> GMNLANIV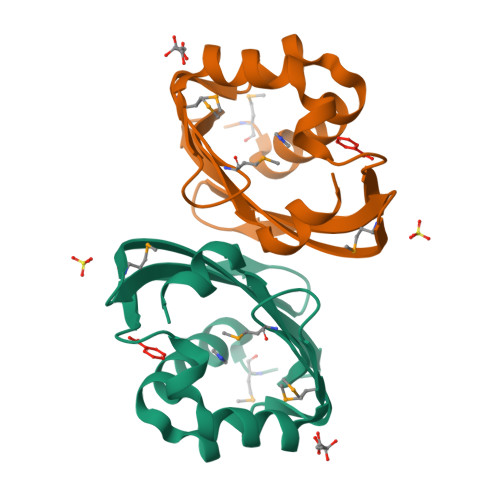QRGWEALGAGDFDTLVTDYVEKMIFIMPGQADVLKGRQAFRSALDNLGEILPPGFEITGLRQLEGENEIVSIVEWKSDKMIASQLSVLFKFEGDQIYEERWFVDTEQWKSVF>SGQNYPEEADGTLDCISMALTCTFNRWGTLLAVGCNDGRIVIWDFLTRGIAKIISAHIHPVCSLCWSRDGHKLVSASTDNIVSQWDVLSGDCDQRFRFPSPILKVQYHPRDQNKVLVCPMKSAPVMLTLSDSKHVVLPVDDDSDLNVVASFDRRGEYIYTGNAKGKILVLKTDSQDLVASFRVTTGTSNTTAIKSIEFARKGSCFLINTADRIIRVYDGREILTCGRDGEPEPMQKLQDLVNRTPWKKCCFSGDGEYIVAGS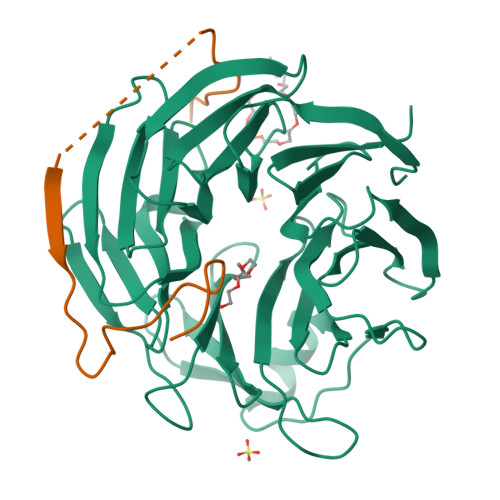ARQHALYIWEKSIGNLVKILHGTRGELLLDVAWHPVRPIIASISSGVVSIWAQNQ[2x];>DEELEDSKALLYLPIAPEVEDPEENPYGPPPDGSQPPKKKPKTTNIELQGVPNDEVHPLLGVKGDGKSK[2x]>SNAMLQKINRYTHGFVAVPVILACREKGVFELLADESPLSLNQMVEHLGANSGHFQVALRMLESLHWLSRNKELKYSLTAEAAIHNKISEDILQLYNLPIQSYLEGKQGNLLGRWIERSCQLWNLDNPLMADFLDGLLVIPLLLALHKHNLLADSEDKPLLSSLSSTVQEELGKLFLHLGWADLTAGRLTITELGRFMGERALNTAIVASYTPMLSRIHDVLFGNCLSVFQRDASGHERHIDRTLNVIGSGFQHQKYFADLEESILSVFNQLPLEEQPKYITDMGCGDGTLLKRVWETIQFKSARGKALEQYPLRLIGVDYNEASLKATTRTLASLPHLVLQGDIGNPEQMVRSLEAHGIHDPENILHIRSFLDHDRLFIPPQKRNELKERAHLPYQSVCVDDQGELIPPHVMVQSLVEHLERWSQVVNKHGLMILEVHCLEPRVVYQFLDKSENLHFDAHQGFSQQYLVEAEVFLMSAAQVGLFPKLELSKRYPKTFPFTRITLNYFEKRPYKISHAYLSDLPALVDLEVKCWPENLRASTHEIRRRLELNPQGNLVLIIEDQIIGAIYSQTITSTEALENVKYAQVPTLHTPQGSVIQLLALNILPEFQARGLGNELRDFMLYYCTLKGGIESVVGVTRCRNYVNYSQMPMMEYLKLHNEQRQLLDPIVGFHVSGGAEIRGIIANYRPEDTDNLGMGILIEYNLRDSALHS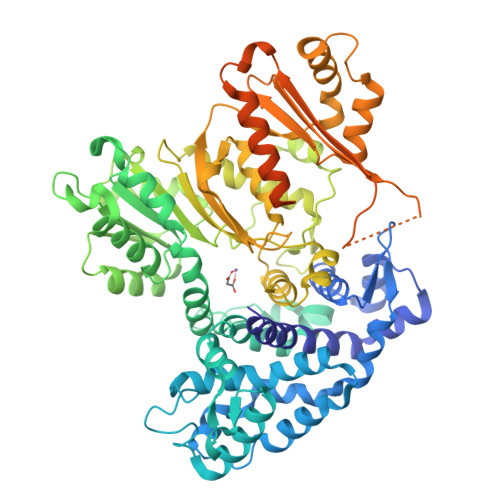[2x]> MKVIFL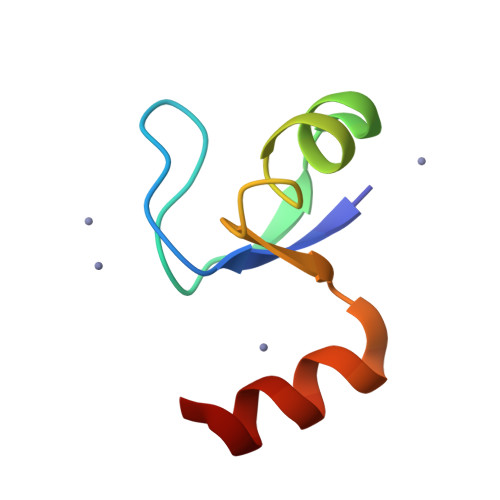KDVKGKGKKGEIKNVADGYANNFLFKQGLAIEATPANLKALEAQK4-[3-(1-methylpiperidin-4-yl)-1,2,4-oxadiazol-5-yl]phenol 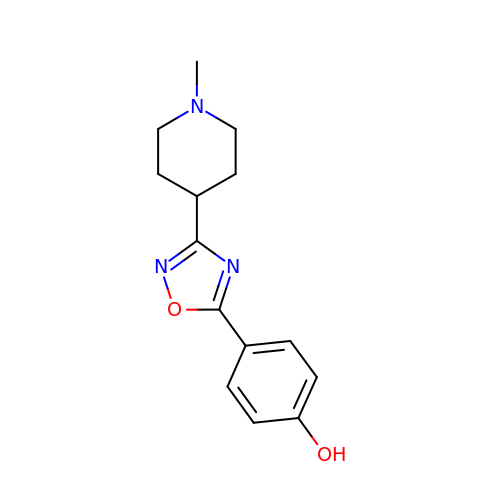| C14 H17 N3 O2 | BGJREFNVLIBEOU-UHFFFAOYSA-N>MEGGMEKGTFQIKTGFAEMFKGGVIMDVTTPEQAVIAEEAGAVAVMALERVPADIRAQGGVARMSDPKIIKEIMAAVSIPVMAKVRIGHFVEAMILEAIGVDFIDESEVLTPADEEHHIDKWKFKVPFVCGARNLGEALRRIAEGAAMIRTKGE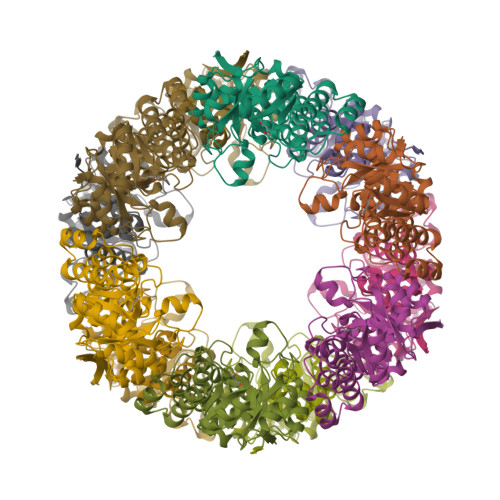AGTGNVVEAVRHARTMWKEIRYVQSLREDELMAYAKEIGAPFELVKWVHDHGRLPVVNFAAGGIATPADAALMMHLGMDGVFVGSGIFKSGDPRKRARAIVRAVAHYNDPEVLAEVSEDLGEPMVGINLDQLKEEERLAKRGW[4x]> MEDITSGLKQLDSTYQETNQQVLKNLDEIFSTTSPSANNEMGEEDALNIKKAAIALRGDLALLKANFEANELFFISEDVIFKTYMSSPELLLTYMKINPLDQNTAEQQCGISDKVLVLYCEGKLKIEQEKQNIRERLETSLKAYQSNIGGTASLITASQTL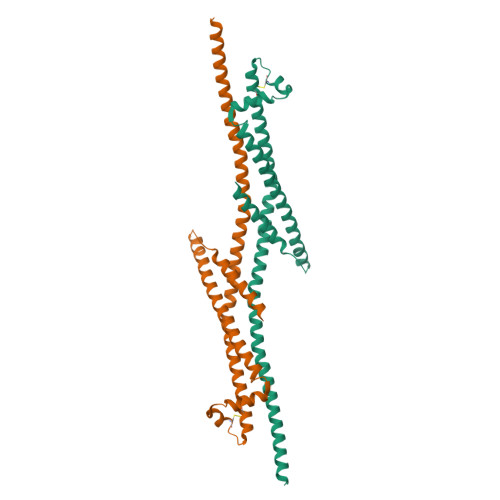VESLKNKNFIKGIRKLMLAHNKVFLNYLEELDALERSLEQSKRQYLQERQSSKIIVKLEHHHHHH>MKIQAGQLGLDDNDVPGPLPDTDSKPSSQSQNDTPMFKLGNFESPVLKELSRRTVNKEMETQRIMTNVIAFAFWNLLVKFIKFFWNNTHVGRQFCNRLSRIHLYMLTFHTLKKANIIYHTTFSWLNAELLDYLFHLLISLNILFSLWKLLSTVKVSDLNLTDRQKKLLGVDMQSSVDTGLQPQHPHYVSTSKISQMAQNKTHIPQTNLKNHPAYLFKGLETPLKARQREMAEEQTKLQSQSLHTKNVFGTLQRHSGISSTLVSANNDNNSPHTPVTRKGYIPSSKYAYMMNSQSPRGKI[2x];>[2x]MEHRYNVFNDTPRGNHWMGSSVSGSPRPSYSSRPNVNTTRRFQYSDDEPAEKIRPLRSRSFKSTESNISDEKSRISERDSKDRYINGDKKVDIYSLPLISTDVLEISKQRTFAVILFLIIQCYKIYDLVILKSGLPLSGLLFKNYRFNFISKYFIIDSFFLYVLPSFNIPRLTFKPWVVYLQILAMLLLNIFISSDHEFVLISLIMTTWRKLYTKELSVTGSAINHHRIFDSSAHFKGALTIKILPENTAMFNPLHESYCLPMDTNLFKINSIDVPIRINSTEEIEYIELEYRDLYTNSVELRSLSKKDFKIIDNPKSFLKKDQSVLKSHSNDFEEGSTIRYLAVTLQDIGFYQIKKIVDSKKLNLKIHQSHLVVPYCPIASITGTGSNDRCIGDSDNVSFEIQGVPPMKLAYSKIVNGQTFSYVDSSLQPEYFESPLQSSKSKQSFTQGELNDLKWGRNQPVNINLDSSITQDGKFAYKIDKITDGLGNVVDFTSLPEELKKRYDLSYNFNVHEVPRAALEERFDPKSPTKRSIAIVFEEIKN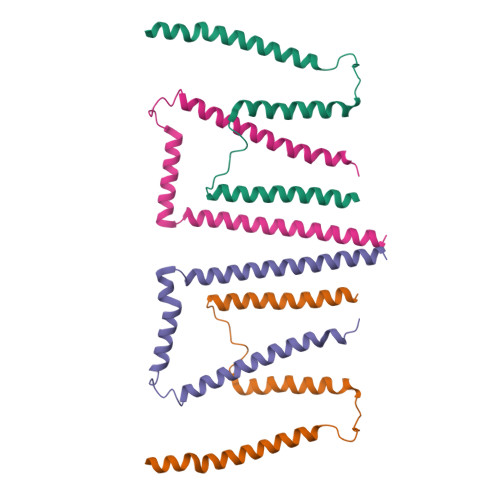WISDIPYVISLSYTDAQDKSKKIMNVTTDSLTKVLQADLPGSYNLEYIESKFCPGEIVGKSNVLVTMPVAPTMEVKSFPILDQCVGQVGLNFELSFTGAPPYYYNTKIYKLENGERKLYDAKRYTSEGTRNRFSYSPPKEGNYEIVFDTVSNKLFTEPIKLEPVKEYTFKTSMRVKPSASLKLHHDLKLCLGDHSSVPVALKGQGPFTLTYDIIETFSSKRKTFEIKEIKTNEYVIKTPVFTTGGDYILSLVSIKDSTGCVVGLSQPDAKIQVRRDIPSAAFNFFEPIKEAKIKHGSVTEIPLKLSGEGPFTVKFKHMDYDGNIVKEFENKFQNSYKPALKVSKEGLYQLVDIRDSSCQGNVIYRNSLYKVSFLEKPKFAIQDNHHITKVTENLFSKEEVCQGMEGTVDLALFGSPPFILEYDLMAPNGHISTKKIQVATKYASLKLPNQIPGEYITTIKAIFDGNYGESDIHFREHQSELIIKQTVHPIPDVAFADGGKTLRACAANVDQISFLEPINLKFLQGESPFSITFSVYHESTSRTDQYTIDNIDSENFSFEKLYEGMKLGNHAITIDSVVDANGCVNSLISGPRNQILVSITDAPKIHILDPSTEYCVGDYVAYQLNGVAPFMIKYEFNGIPLKSKERSSQFVRLASEPGIISITSLQDSSSQCIVDFTNPKLKSEFDDLSLNIHPIPSVTVSQGNYVTEDIREGDQAEVIFSFEGTPPFSLTYVRTEETDGKHGKRRSQVVETHKVTDIYSHEYKVITSLQGTYEAIEITDAYCFAKNDLFFNN>[3x]GPGSMGTVTTKDGVEIFYKDWGPRDAKVIHFHHGWPLSSDDWDAQLLFFVNKGFRVVAHDRRGHGRSSQVWDGHDMDHYADDAAAVVEKLGTHGAMHVG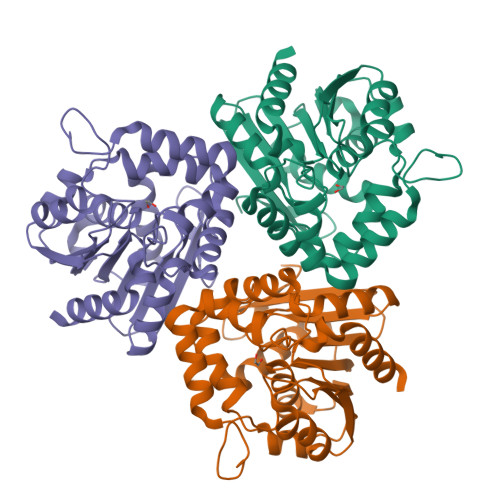HSTGGGEVVRYIARHGERNVSKAVLISSVPPLMVKTSSNPNGTPKSVFDDFQAHVAANRAQFYLDVPAGPFYGYNRPGAKPSEGVIYNWWRQGMMGSTKAQYDGIVAFSQTDFTNDLKGITIPVLVIHGDDDQVVPYADSGVLSAKLVKNGKLITYKGAPHGIPTTHADKVNADLLEFLQS> GP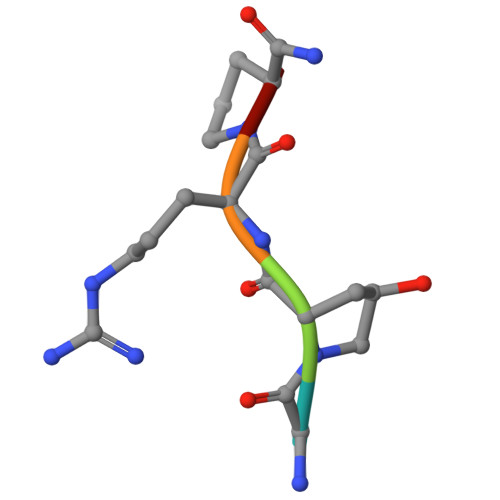RPX> PYVEITEQPHPKALRFRYECEGRSAGSIPGVNTTAEQKTFPSIQVHGYRGRAVVVVSCVTKEGPEHKPHPHNLVGKEGCKKGVCTVEINSTTMSYTFNNLGIQCVKKKDVEEALRLRQE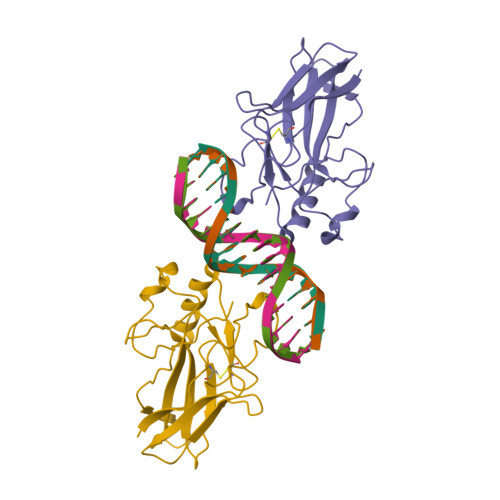IRVDPFRTGFGHAKEPGSIDLNAVRLCFQVFLEGQQRGRFTEPLTPVVSDIIYDKK2-(butylamino)quinolin-8-ol | C13 H16 N2 O | 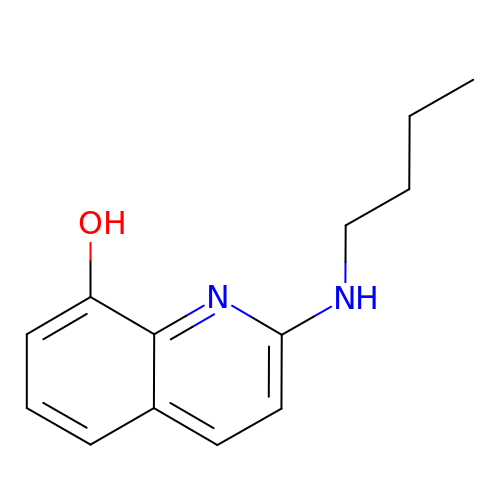JEHFWPXGFVJHCI-UHFFFAOYSA-N>VKAIWADPKEVHDAGGISVGDRWKALANALNIPLDQLSARINANPKGRFIYLARQVNPDMADYIKKLKLPGIHLREES[8x]

The penicillin-binding proteins (PBPs) synthesize and remodel the cell wall peptidoglycan, a major component of the bacterial cell wall that gives the cell its shape and rigidity. In E. coli, PBP3 (FtsI) is an essential protein of the divisome, catalyzing peptide cross-bridges between the glycan chains of the peptidoglycan. The overall fold of periplasmic PBP3 is bimodular. The C-terminal module is responsible for the transpeptidase activity but no clear function has been assigned yet to the N-terminal module of the construct.

In order to determine its three-dimensional structure, the PBP388–165 domain was produced and its structure solved. The domain crystallizes in P1 with eight molecules in the asymmetric unit. The structure of the PBP388–165 domain was eventually determined by single anomalous diffraction using a selenomethionine substituted PBP388–165 crystal and refined over data collected on a crystal of the native PBP388–165 protein. The eight molecules in the asymmetric unit are organized in four pairs with, in each pair, 18 N-terminal residues swapping into the paired molecule. The swapped residues represent a two-turn helix and a β-strand that inserts between two β-strands of the other molecule to form a three stranded β-sheet. Interactions between the two molecules are numerous and include many hydrogen bonds, salt bridges (e.g. for associated chains A and C: Asp94A-Arg135C, Glu97A-His160C), hydrophobic clusters (Ile91A is surrounded by seven leucines or isoleucines from chain C), and an aromatic ring stacking (Trp92A is sandwiched between Phe136C and His160C). Together, residues 88–105 from one molecule and residues 106–165 from the paired molecule form a small globular domain whose tertiary structure, three anti-parallel β-strands flanked by three helices, is homologous to the equivalent domain of P. aeruginosa PBP3. DLS and SLS experiments carried out on a solution of PBP388–165 suggested a dimer in solution. From these results, we conclude that, at the concentration used for crystallization, monomers of PBP388–165 are absent and dimers are predominant in the solution. The structure of the PBP388–165 domain, disordered in PBP3, shows a dimerization of the domain by three dimensional domain swapping that is possible but unlikely in the full length PBP3.N-{5-[difluoro(phosphono)methyl]-1-benzothiophene-2-carbonyl}-3-methyl-L-valyl-L-prolyl-N,N-dimethyl-N~3~-[4-(1,3-thiazol-2-yl)phenyl]-beta-alaninamide 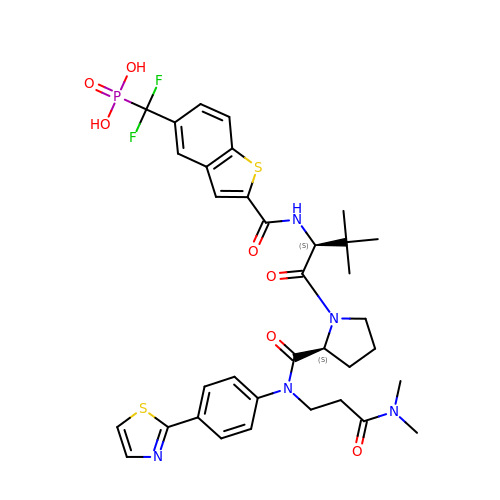| C35 H40 F2 N5 O7 P S2 | KJJHAYNANYPNEE-ABYGYWHVSA-N Human bestrophin1 (hBest1) is a Ca2+-activated Cl− channel essential for Cl− transport in retinal pigment epithelium (RPE). Although the structure of hBest1 is still unsolved, two Best1 homolog structures, one from bacteria Klebsiella pneumoniae (KpBest) and the other from chicken (cBest1), have been previously reported. Overall, the channel is a pentameric assembly with a single ion-conducting pathway, which varies in diameter along its length and is constrained at two narrow points: a “neck” contributed by three residues (I62/I66/F70 in KpBest and I76/F80/F84 in hBest1/cBest1) on a transmembrane helix, and an “aperture” formed by a single residue (I180 in KpBest1, I205 in hBest1, and V205 in cBest1) on a cytosolic helix. Here, by electrophysiological and structural analyses, we show that the neck and aperture in hBest1 are both indispensable Ca2+-dependent gates, and their dysregulated opening by rationally designed or patient-derived mutations causes Ca2+-independent leak and elevates Ca2+-dependent channel activity.

Alanine substitution mutants for each of the 12 residues were generated in KpBest and hBest1 and subjected to crystallography and patch clamp, respectively. Moreover, the equivalent KpBest mutants (W16A, G18A, S19A, L259A, P262A, G264A, and D269A) all showed an overall similar structure to that of WT KpBest. The corresponding “Ca2+-binding” sites in WT KpBest are occupied by Zn2+, an essential component in the crystallization buffer. Interestingly, the KpBest P262A, G264A, and D269A mutants show no Zn2+ in the corresponding sites. Moreover, KpBest L259A, P262A, G264A, and D269A all have relatively low resolution and slightly altered structures in this region, suggesting that the binding of Zn2+ stabilizes the channel structure.

>[5x]NAMIIRPEQHWFLRLFDWHGSVLSKIIFRLLLNVLMSIIAIISYQWYEQLGIHLTVAPFSLLGIAIAIFLGFRNSASYSRFVEARNLWGTVLIAERTLVRQLRNILPAEHDAHRRIVSYLVAFSWSLKHQLRKTDPTADLRRLLPEERVTEILASSMPTNRILLLAGNEIGQLREAGKLSDITYGLMDNKLDELAHVLGGCERLATTPVPFAYTLILQRTVYLFCTLLPFALVGDLHYMTPFVSVFISYTFLSWDSLAEELEDPFGTAANALPLNAMCNTIERNLLDMTGQHPLPE>[2x]MHEYELNQDLLAENKRLAEKNREALRESGTVAVNIMGAIGSGKTLLIERTIERIGNE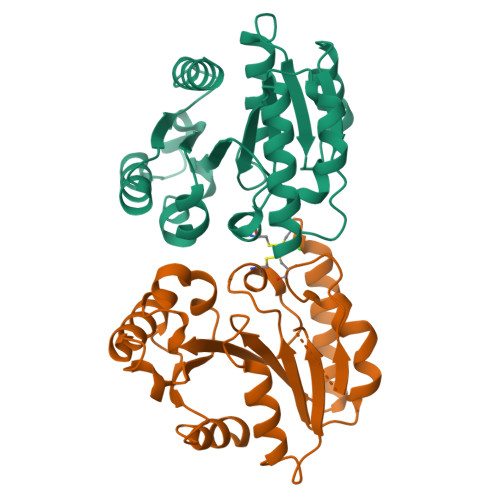VKIGAMLGDVVSKADYERVRRFGIKAEAISTGKECHLDAHMIYHRLKKFSDCDLLLIENVGNLICPVDFDLGENYRVVMVSVTEGDDVVEKHPEIFRVADLIVINKVALAEAVGADVEKMKADAKLINPRAKIIEMDLKTGKGFEEWIDFLRGILNVHSDSGQN>MGSSHHHHHHSSGLVPRGSHSQPSTANGGFPSVVVTAVTATTSISPDIESTWKGLLAGESGIHALEDEFVTKWDLAVKIGGHLKDPVDSHMGRLDMRRMSYVQRMGKLLGGQLWESAGSPEVDPDRFAVVVGTGLGGAERIVESYDLMNAGGPRKVSPLAVQMIMPNGAAAVIGLQLGARAGVMTPVSACSSGSEAIAHAWRQIVMGDADVAVCGGVEGPIEALPIAAFSMMRAMSTRNDEPERASRPFDKDRDGFVFGEAGALMLIETEEHAKARGAKPLARLLGAGITSDAFHMVAPAADGVRAGRAMTRSLELAGLSPADIDHVNAHGTATPIGDAAEANAIRVAGCDQAAVYAPKSALGHSIGAVGALESVLTVLTLRDGVIP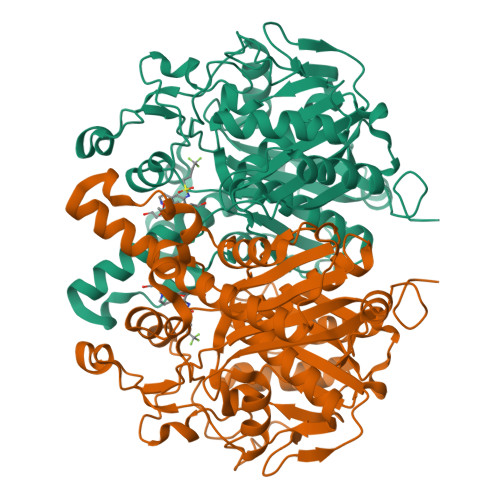PTLNYETPDPEIDLDVVAGEPRYGDYRYAVNNSFGFGGHNVALAFGRY[8x]> M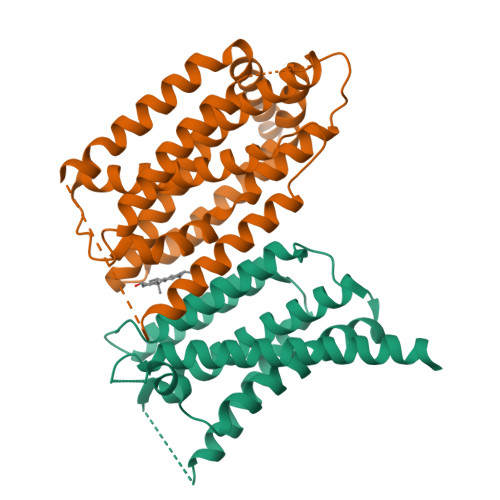AEGETESPGPKKSGPYISSVTSQSVNLMIRGVVLFFIGVFLALVLNLLQIQRNVTLFPPDVIASIFSSAWWVPPCCGTASAVIGLLYPSIDRHLGEPHKFKREWSSVMRCVAVFVGINHASAKVDFDNNIQLSLTLAALSIGLWWTFDRSRSGFGLGVGIAFLATVVTQLLVYNGVYQYTSPDFLYVRSWLPCIFFAGGITMGNIGRQLAMYESKVIAEKSHQE;> MTLTERLREKISRAFYNHGLLCASYPIPIILFTGFCILACCYPLLKLPLPGTVPGKYSGVSLYTRKRMVSYTITLVFQHYHAKFLGSLRARLMLLHPSPNCSLRAESLVHVHFKEEIGVAELIPLVTTYIILFAYIYFSTRKIDMVKSKWGLALAAVVTVLSSLLMSVGLCTLFGLTPTLNGGEIFPYLVVVIGLENVLVLTKSVVSTPVDLEVKLRIAQGLSSESWSIMKNMATELGIILIGYFTLVPAIQEFCLFAVVGLVSDFFLQMLFFTTVLSIDIRRMELADLNKRLPPEACLPSAKPVGQPTRYERQLAVRPSTPHTITLQPSSFRNLRLPKRLRVVYFLARTRLAQRLIMAGTVVWIGILVYTDPAGLRNYLAAQVTEQSPLGEGALAPMPVPSGMLPPSHPDPAFSIFPPDAPKLPENQTSPGESPERGGPAEVVHDSPVPEVTWGPEDEELWRKLSFRHWPTLFSYYNITLAKRYISLLPVIPVTLRLNPREALEGRHPQDGRSAWPPPGPIPAGHWEAGPKGPGGVQAHGDVTLYKVAALGLATGIVLVLLLLCLYRVLCP Coxsackievirus A9 (CVA9) belongs to the Enterovirus genus, species Enterovirus B (EV-B) in the family Picornaviridae. Like other picornaviruses, CVA9 has a small, ~30-nm-diameter, nonenveloped viral capsid. Its positive-sense single-stranded RNA genome is ~7,500 bases long and encodes 4 structural proteins (VP1 to 4) and 7 nonstructural proteins (2A to C and 3A to D). During cell entry, enterovirus capsids undergo conformational changes leading to expansion, formation of large pores, externalization of VP1 N termini, and loss of the lipid factor from VP1.

To evaluate structural changes in the CVA9 virions induced by different treatments, we solved cryo-EM structures of the most populated classes from intact, faf-BSA-treated, and ion-treated CVA9 data sets to 2.9, 3.5, and 3.3 Å resolution, respectively. Similar to the X-ray structure, the intact virion reconstruction showed elongated density for a lipid factor placed in the hydrophobic pocket in VP1, as well as a large portion of the myristoyl (MYR) group covalently attached to the VP4 N terminus. Furthermore, the base-stacking interaction between vRNA and VP2 Trp38 next to the 2-fold axis inside the intact virion could be clearly observed. The average radius of the intact virion, 15.6 nm, coincided well with the geometric radius measured in AF4 experiments. As expected, the main particle population in the control data set was that of intact particles (89%), but there were also expanded particles containing viral genome (5%) and empty nonexpanded capsids observed (6%). In the intact virion, the RNA was tethered to the capsid via the VP2 Trp38, but it also was in close contact all over the capsid interior. SYBR green II interacts with free nonencapsidated RNA, or it can access vRNA due to the pores in the expanded capsids. In Dulbecco’s phosphate-buffered saline (DPBS), the virions were stable for 3 h according to the very low fluorescence readout throughout the measurement (Fig. 1A, black solid line). In the control sample, 8.8% of the spectral counts for the structural proteins corresponded to VP4 (13 spectra out of 134), which agreed well with the stoichiometry-based calculations from the virion amino acid composition, where VP4 accounted for 7.8% of the total.

> GDVEEAIERAVVHVADTMRSGPSNSASVPALTAVETGHTSQVTPSDTMQTRHVKNYHSRSESTVENFLGRSACVYMEEYKTTDNDVNKKFVAWPINTKQMVQMRRKLEMFTYLRFDMEVTFVITSRQDPGTTLAQDMPVLTHQIMYVPPGGPIPAKVDDYAWQTSTNPSIFWTEGNAPARMSIPFISIGNAYSNFYDGWSNFDQRGSYGYNTLNNLGHIYVRHVSGSSPHPITSTIRVYFKPKHTRAWVPRPPRLCQYKKAFSVDFTPTPITDTRKDINTVTTVAQSRRRGDMSTLNTH;> SPTVEECGYSDRVRSITLGNSTITTQECANVVVGYGRWPTYLRDDEATAEDQPTQPDVATCRFYTLDSIKWEKGSVGWWWKFPEALSDMGLFGQNMQYHYLGRAGYTIHVQCNASKFHQGCLLVVCVPEAEMGGAVVGQAFSATAMANGDKAYEFTSATQSDQTKVQTAIHNAGMGVGVGNLTIYPHQWINLRTNNSATIVMPYINSVPMDNMFRHYNFTLMVIPFVKLDYADTASTYVPITVTVAPMCAEYNGLRLAQAQ;> GLPTMNTPGSTQFLTSDDFQSPCALPQFDVTPSMNIPGEVKNLMEIAEVDSVVPVNNVQDTTDQMEMFRIPVTINAPLQQQVFGLRLQPGLDSVFKHTLLGEILNYYAHWSGSMKLTFVFCGSAMATGKFLIAYSPPGANPPKTRKDAMLGTHIIWDIGLQSSCVLCVPWISQTHYRLVQQDEYTSAGYVTCWYQTGMIVPPGTPNSSSIMCFASACNDFSVRMLRDTPFISQDNKLQ;> GAQVSTQKTGAHETSLSAAGNSIIHYTNINYYKDAASNSANRQDFTQDPSKFTEPVKDVMIKSLPALN>[2x]MNLVLMGLP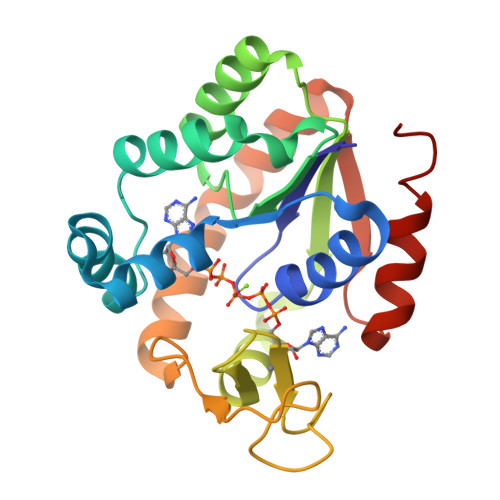GAGKGTLGERIVEDYGIPHISTGDMFRAAMKEETPLGLEAKSYIDKGELVPDEVTIGIVKERLGKDDCERGFLLDGFPRTVAQAEALEEILEEYGKPIDYVINIEVDKDVLMERLTGRRICSVCGTTYHLVFNPPKTPGICDKDGGELYQRADDNEETVSKRLEVNMKQTQPLLDFYSEKGYLANVNGQRDIQDVYADVKDLLGGLK D-MANNITOL-1,6-DIPHOSPHATE 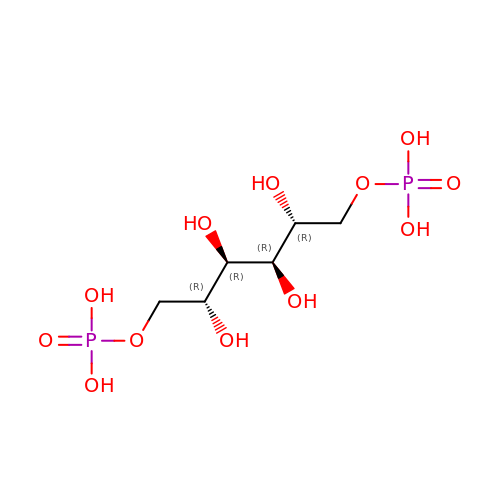| C6 H16 O12 P2 | WOYYTQHMNDWRCW-KVTDHHQDSA-N> MKLTIIRLEKFSDQDRIDLQKIWPEYSPSSLQVDDNHRIYAARFNERLLAAVRVTLSGTEGALDSLRVREVTRRRGVGQYLLEEVLRNNPGVSCWWMADAGVEDRGVMTAFMQALGFTAQQGGWEKCSGLE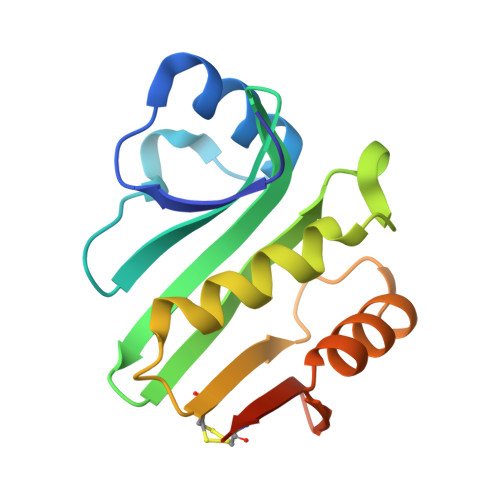HHHHHH UdgX excises uracil from uracil-containing DNA to concurrently form a covalent bond with the resulting AP-DNA. Structurally, UdgX is highly similar to family-4 UDGs (F4-UDGs). However, UdgX is unique in possessing a flexible R-loop (105KRRIH109). Our earlier studies allowed us to propose a reaction mechanism of UdgX, which involves the formation of a covalent bond between H109 of UdgX with the C1′ position of the target deoxyribose sugar concurrently with the uracil excision from this site in DNA.

It possesses α/β/α fold with four central parallel β stranded sheet sandwiched between the α helices. The functionally important elements such as motif A, motif B, and the R-Loop sequences of MsmUdgX, and the conserved sequence 90TNAV93 found in UDGs are shown in Figures 1A and B. UdgX follows a unimolecular substitution (SN1) reaction mechanism, wherein the glycosidic bond between uracil and the deoxyribose sugar in the DNA is replaced by a unique His-deoxyribose sugar covalent bond (1.5 Å) in UdgX–DNA upon excision of uracil. Briefly, as a first step in the reaction, uracilate anion formation is facilitated by hydrogen bonding of H178 and N91 with the uracil in the active site pocket, resulting in a ‘pulling’ force on uracil and weakening of the glycosidic bond. In the next step, E52 (motif A) activates the H109 (R-Loop), converting it into an efficient nucleophile to facilitate its covalent bonding with C1′ (having a positive charge imparted upon it by departure of uracilate anion) of the target deoxyribose sugar. Q53 makes hydrogen bonds with the O of K110 (2.87 Å) and N of K97 (2.82 Å). These interactions remain intact in the DNA bound form with bond distances of 2.69 and 2.79 Å, respectively. Thus, these interactions may help anchor the R-loop towards the active site of UdgX. Our studies suggest a major role of H109 in carrying out the unique role of UdgX in forming a covalent bond appears to be facilitated by its ability in avoiding a water molecule in this location, whose activation by E52 would otherwise result in the release of the AP-DNA, as in other UDGs.

> AGAQDFVPHTADLAELAAAAGECRGCGLYRDATQAVFGAGGRSARIMMIGEQPGDKEDLAGLPFVGPAGRLLDRALEAADIDRDALYVTNAVKHFKFTRAAGGKRRIHKTPSRTEVVACRPWLIAEMTSVEPDVVVLLGATAAKALLGNDFRVTQHRGEVLHVDDVPGDPALVATVHPSSLLRGPKEERESAFAGLVDDLRVAADV> MSMLVVVTENVPPRLRGRLAIWLLE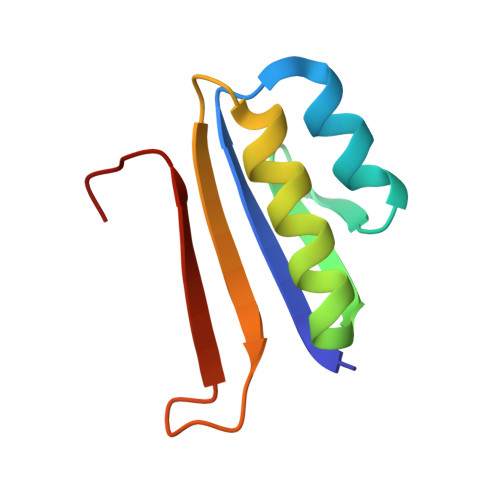VRAGVYVGDVSAKIREMIWEQIAGLAEEGNVVMAWATNTETGFEFQTFGLNRR The flavoprotein FerB (ferric reductase B, a product of gene 4071) was originally isolated from the cytoplasm of the soil bacterium Paracoccus denitrificans as one of two major enzymes able to reduce Fe(III)-ligand complexes when NADH was the electron donor. The protein is also active as a chromate reductase and, to a substantially greater extent, as a quinone reductase. There is an expanding list of bacterial flavoenzymes that display redox activities against diverse xenobiotics, such as heavy metal ions like chromate, nitro compounds, azo dyes and carbonyl compounds including quinones. These enzymes occur as homodimers or homotetramers with a non-covalently bound flavin mononucleotide (FMN) cofactor and display a bi-bi ping-pong mechanism with NAD(P)H as the presumed physiological reductant. For this, the crystal structure of holoenzyme has been solved and the effect of mutating the strategically selected residues has been analyzed by means of fluorimetric titration of free flavin by apoenzyme, enzyme kinetic assays and spectropotentiometry.

The crystals belong to the orthorhombic space group P21212 with two protein molecules in an asymmetric unit. The final model contains residues 2-182 (monomer A and B), one polyethylene glycol fragment, 451 water molecules and two flavin adenine mononucleotides. Each monomer has an α/β twisted open-sheet structure containing alpha helices on both sides of the central β-sheet in an arrangement typical for a flavodoxin-like fold. Five parallel strands in the order β2, β1, β3, β4, β5, are sandwiched between the helices α1 and α5 on one side and the helices α2, α3 and α4 on the other side. The two molecules of the asymmetric unit form a head-to-tail homodimer with two symmetrical active sites facing the opposite sides and located at the interface between the subunits. Dimerization occurs mainly via anti-parallel packing of helices α3 and α4 into a four-helix bundle. Contrary to the initial experimental hints, the present X-ray crystal data show unequivocally that FMN and not FAD is a true cofactor of FerB. The isoalloxazine ring of FMN in enzyme crystal is bent 12.8° along the N5-N10 axis. It is uncertain at present whether the initially planar oxidized isoalloxazine adopted this conformation as a result of binding to protein or whether it was only later converted to a bent semiquinone by photoelectrons generated during data collection. The FMN binding site is mainly composed of residues from the loops L1 and L3, supplemented by a few residues belonging to the adjacent subunit (Tyr46, Asp48, Arg95).

>MVKTVAVMVGSLRKDSLNHKLMKVLQKLAEGRLEFHLLHIGDLPHYNDDLWADAPESVLRLKDRIEHSDAVLAITPEYNRSYPGMIKNAIDWATRPYGQNSWKGKPAAVIGTSPGVIGAALAQARLKNDLLHVGTVMMSMPEAYIQWHAEAYAADGSVTDEKTAKFLQGFVDAFVDWIEKHGLEHHHHHH[2x]>MLPFATIPATERNSAAQHQDPSPMSQPFDLPALASSLADKSPQDILKAAFEHFGDELWISFSGA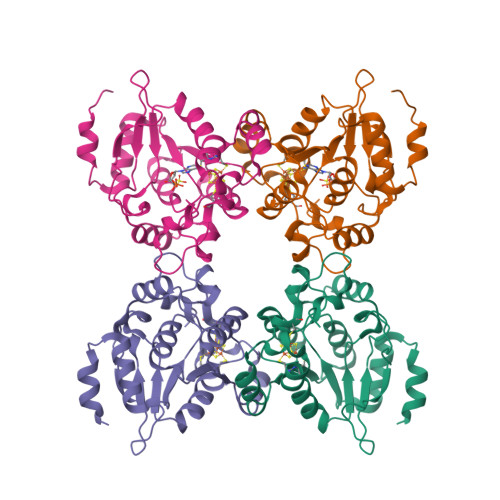EDVVLVDMAWKLNRNVKVFSLDTGRLHPETYRFIDQVREHYGIAIDVLSPDPRLLEPLVKEKGLFSFYRDGHGECCGIRKIEPLKRKLAGVRAWATGQRRDQSPGTRSQVAVLEIDGAFSTPEKPLYKFNPLSSMTSEEVWGYIRMLELPYNSLHERGYISIGCEPCTRPVLPNQHEREGRWWWEEATHKECGLHAGNLISKALEHHHHHH[8x]> MEPPFEWSPQFILLLLAVTTYGFPLEEKFDGLFRAEPPHCSKTPIVRAQTSQNAMSSIARGMQMQFSIGLHTAVCFRLYEDTQLASQEINDDENAGNQTSLLHTIRLEKLEHHHPITQRYTFGIPEVHASCICECDATSSTCTAESHQFTACPESDKSDETSSCYRTFFPNQTPIGCSEDDIPKLCCDVRFKPYKNMTFLAVKLEQPTTYATFVYAAYDFVNGYWVEKDKTKIRSQLDGGTQDRHLDQKRRISLAVTAGGRASHQLETGMYFSRTSNGGETEELRMQPLNEITDNNFDRLGWYRMDDSGHFHVNNGVVKMDDIHKAKVKNCKEQTYKSILSANHYMPGHFNLTRPLEVIKPWIQSARIFDSSLRQAVVTHAEGTNLQISIHLDDEVESQNLVFFHNASRIRDFSGSIIVDSKSNRLFNLTVYEASGKIDGSVKMSTGFGSDTIHTFTAYVSDLHASNRSMIIPLPAIVGQGARAICLRADSMADIDKICHVIEYFESPLEIDLVEGKWHEMIGTCPTCNQINFNGMMKFLNPAHWIKGISSIGDGVMIATDIVVYLGVLCILYLLITKIIVPLVRCWVCPMSIFCNGSSSSSKNKNDKRRKEREERRRKDKFVSESEDGARSSSEPHDTLARYHGNHSERHYSSSQYI

Specific membrane proteins, called fusogens, are required to modulate lipid-bilayers and thereby facilitate membrane merging. The founding members of this cell–cell fusion family (FF) are the epithelial fusion failure 1 (EFF-1) and the anchor-cell fusion failure 1 (AFF-1) proteins, both of which are named after their respective knockout phenotypes. Both proteins have been shown to be sufficient to fuse cells in vivo, and induce fusion of insect and mammalian cells in cell culture when expressed ectopically. FF-mediated fusion appears to be bilateral and homotypic, that is, dependent on the presence of FF proteins on both fusing membranes.

The consistency of EFF-1 proteins on the more spherical vesicles allowed tomogram sub-volumes to be averaged to produce a 3D reconstruction of membrane-anchored EFF-1. Our 3D reconstruction reveals that the natively membrane-anchored ectodomain of EFF-1 has an asymmetric elongated shape. It is ~13 nm long and the region most distal to the membrane (‘head’) has a cross-section of ~6 × 4 nm2. A narrower region (‘tail’) leads to the membrane. The ectodomain of EFF-1 observed in the crystal structure is in the post-fusion trimeric conformation, whereas the native membrane EFF-1 structure determined in this study is monomeric. A protomer from the EFF-1 crystal structure was first fitted as one rigid body into the determined EFF-1 EM reconstruction and gave an overall good fit with a cross correlation coefficient of 0.497. To further improve this fit, the protomer was subjected to four iterations of flexible fitting using Flex-EM25, with each domain considered a rigid body and flexibility allowed only in the hinge regions. Our structure and the fitting unambiguously revealed that domains I and III are distal to the membrane, and that domain II is proximal to the membrane. The flexible fitting of the domains yielded a ~16° rotation around the domain I–II hinge relative to the crystal structure and a ~19° rotation around the domain I–III hinge. In this conformation, the distance between Glu 245 on domain II and Lys 400 on domain III is substantially shorter than in the EFF-1 crystal structure (reduced from ~12 to ~4 Å), suggesting a possible electrostatic connection.Dolichylphosphate | C55 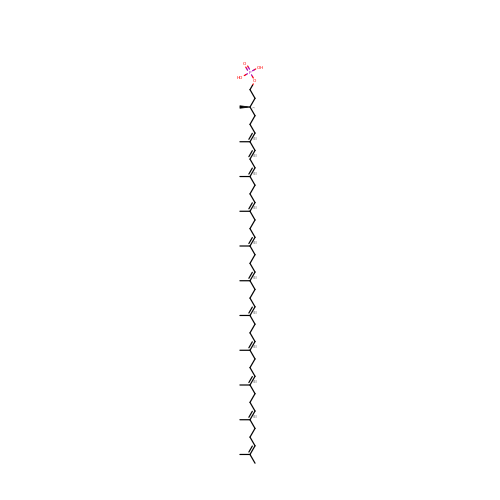H91 O4 P | RELQHJGBFDNPMD-MJTCBKSFSA-N> GSAHGPSAMVFTVIQGSGEPTDTVLRATTLSCAYTAEGTHPAPRAACDALNATDGELNRLLAAPDPSLVCPMYFD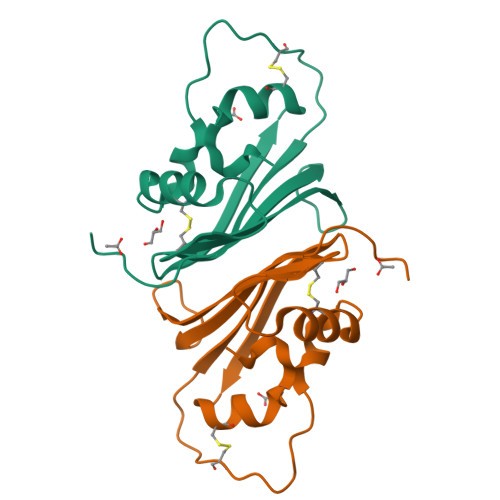PVTVTADGVLNGRRVAWKHTFSNTCVMSANLNSNPVYAF> MGEQVVKPTDERIIDPSTANTQLTGGVCYNTTSGGNKPLAGSPYGYETWIDTGGGVCSLCWYGADQGGGAAFRATWTNPHDFLGRLGYFWNENKPYSHYENIYCGFNYTRSGRKTAGDYSYIGIYGWSRNPSASNSNERLIEYYIVEDWFGNQWQADTSPMGINTTGGT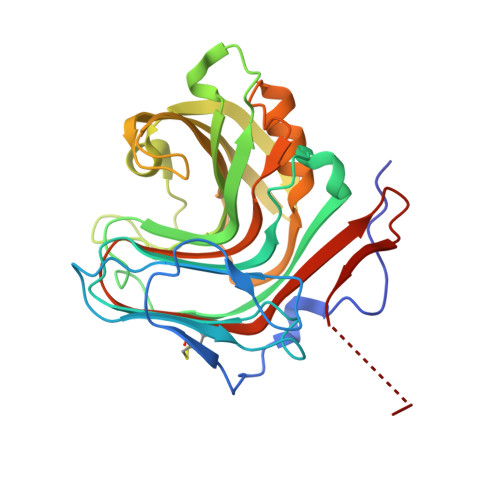VMGSFTVDGSSYQIIRNTRVNQPSIEGDKTFVQYFSIRQSPRKSGTISITEHFKKWEKLGMKLGDNMYECKFLIEAGAGEGFFDARLIQFYRADNEGNILQITPLEHHHHHH>MAPAPPANSGESSLLSESELPAGISYAEAMEGGSRPLLHPDNPVVFFDISIGSHEAGRIKIELFKNLAPKSAENFRQFCTGEFRQNQVPIGYKGATFHRIIKNFMIQGGDFVKGDGTGRLSIYGSSFPDEAFVLPHFRSGLLSLANSGPDTNGCQFFITCAKCDWLNRKHVVFGQVLGKESMQVVRKIEHVTVDGGNRPR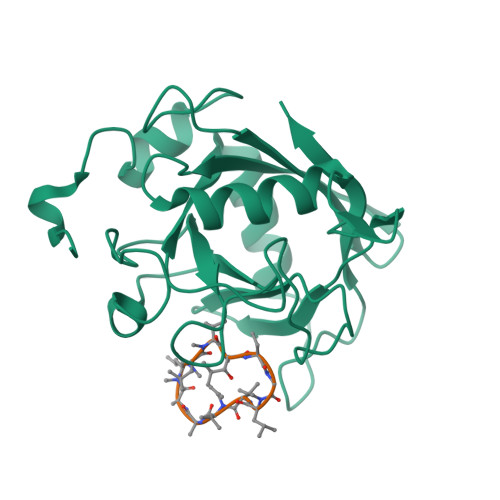IPVTVTQCGEL[2x];>[2x]ALLVTAGLVLA> ASMQKLINSVQNYAWGSKTALTELYGIANPQQQPMAELWMGAHPKSSSRITTANGETVSLRDAIEKNKTAMLGEAVANRFGELPFLF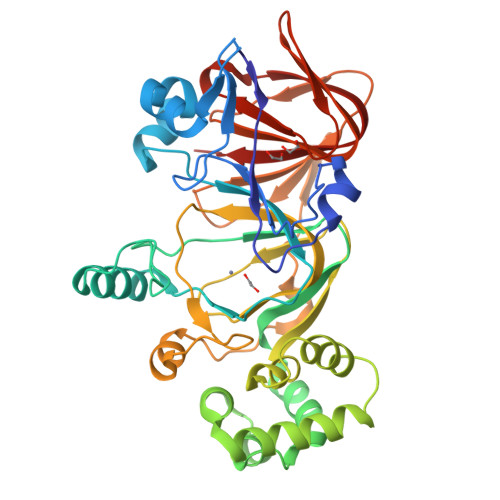KVLCAAQPLSIQVHPNKRNSEIGFAKENAAGIPMDAAERNYKDPNHKPELVFALTPFLAMNAFREFSDIVSLLQPVAGAHSAIAHFLQVPNAERLSQLFASLLNMQGEEKSRALAVLKAALNSQQGEPWQTIRVISEYYPDDSGLFSPLLLNVVKLNPGEAMFLFAETPHAYLQGVALEVMANSDNVLRAGLTPKYIDIPELVANVKFEPKPAGELLTAPVKSGAELDFPIPVDDFAFSLHDLALQETSIGQHSAAILFCVEGEAVLRKDEQRLVLKPGESAFIGADESPVNASGTGRLARVYNKL>MRSRRVDVMDVMNRLILAMDLMNRDDALRVTGEVREYIDTVKIGYPLVLSEGMDIIAEFRKRFGCRIIADFKVADIPETNEKICRATFKAGADAIIVHGFPGADSVRACLNVAEEMGREVFLLTEMSHPGAEMFIQGAADEIARMGVDLGVKNYVGPSVRPERLSRLREIIGQDSFLISPGVGAQGGDPGETLRFADAIIVGRSIFLADNP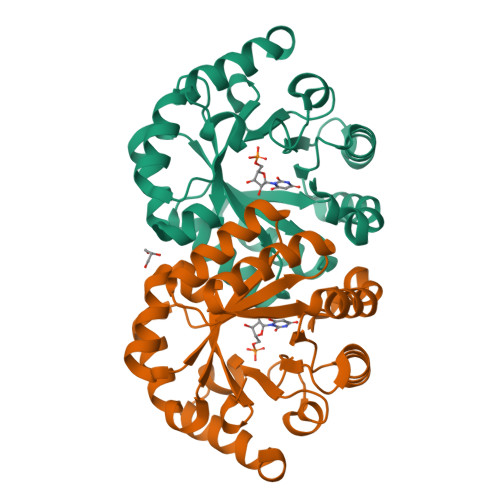AAAAAGIIESIKDLLNP[2x]4-amino-5-hydroxynaphthalene-2,7-disulfonic acid 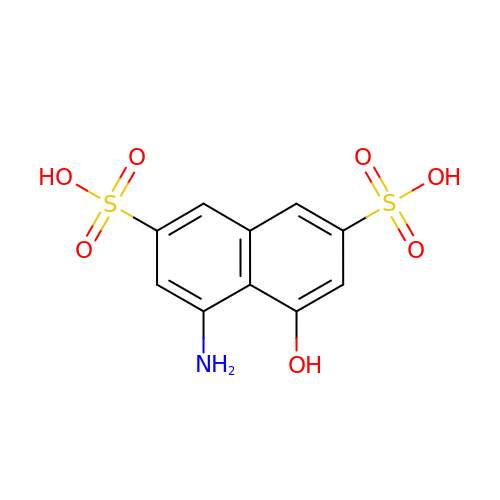| C10 H9 N O7 S2 | APRRQJCCBSJQOQ-UHFFFAOYSA-N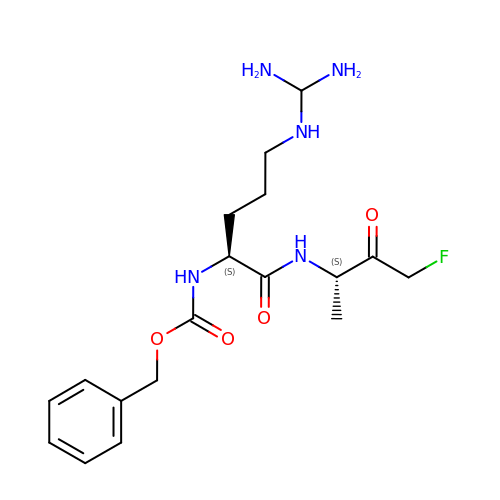BENZOYL-ARGININE-ALANINE-FLUORO-METHYL KETONE | C18 H28 F N5 O4 | FAAPWXRBXXSQNJ-JSGCOSHPSA-N> AAAAAAAA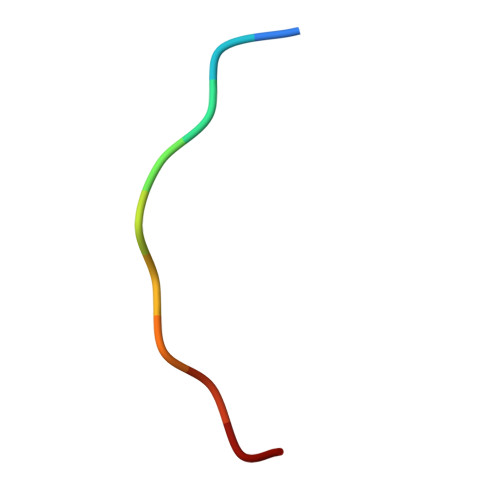AA Estradiol-17beta-glucuronide 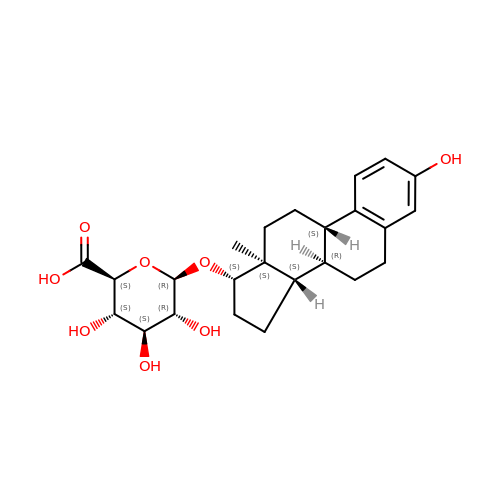| C24 H32 O8 | MTKNDAQYHASLID-QXYWQCSFSA-N> MIRDIIRMGDKRLLRVAPQVTNLGSAELHALVSDMFETMGAAHGVGLAAPQIAV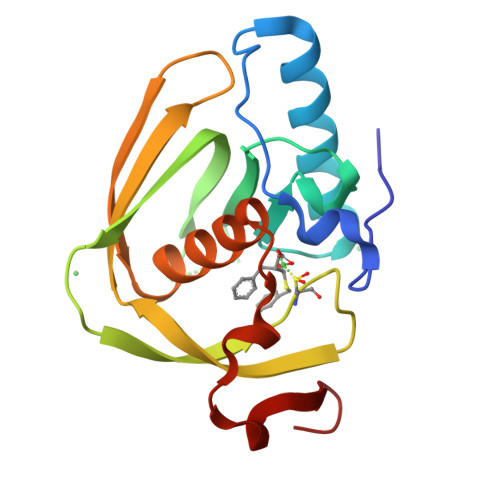DLQLMVFGFEASERYPEAPAVPLTALANAQIEPLSDEMENGWEGCLSIPGLRAVIPRYRYIRYRGFAPDGSPIEREAEGFHARVVQHEYDHLVGRLYPSRIENFDTFGFDDVL>MPTLLRVYIDGPHGMGKTTTTQLLVALGSRDDIVYVPEPMTYWRVLGASETIANIYTTQHRLDQGEISAGD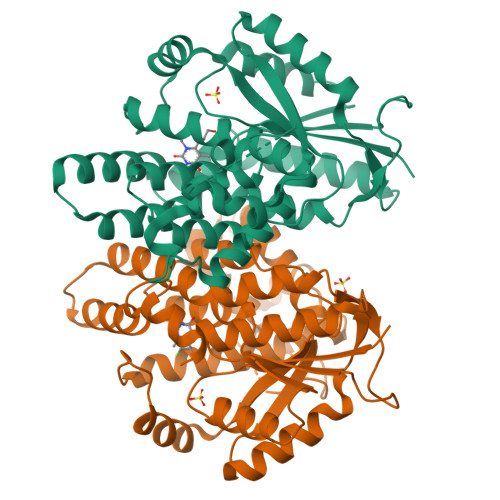AAVVMTSAQITMGMPYAVTDAVLAPHIGGEAGSSHAPPPALTLIFDRHPIAALLCYPAARYLMGSMTPQAVLAFVALIPPTLPGTNIVLGALPEDRHIDRLAKRQRPGERLDLAMLAAIRRVYGLLANTVRYLQCGGSWREDWGQLSGTAVPPQGAEPQSNAGPRPHIGDTLFTLFRAPELLAPNGDLYNVFAWALDVLAKRLRSMHVFILDYDQSPAGCRDALLQLTSGMVQTHVTTPGSIPTICDLARTFAREMGEAN[2x]>[4x]MGSDKIHHHHHHMIDLRSDTVTKPTEEMRKAMAQAEVGDDVYGEDPTINELERLAAETFGKEAALFVPSGTMGNQVSIMAHTQRGDEVILEADSHIFWYEVGAMAVLSGVMPHPVPGKNGAMDPDDVRKAIRPRNIHFPRTSLIAIENTHNRSGGRVVPLENIKEICTIAKEHGINVHIDGARIFNASIAS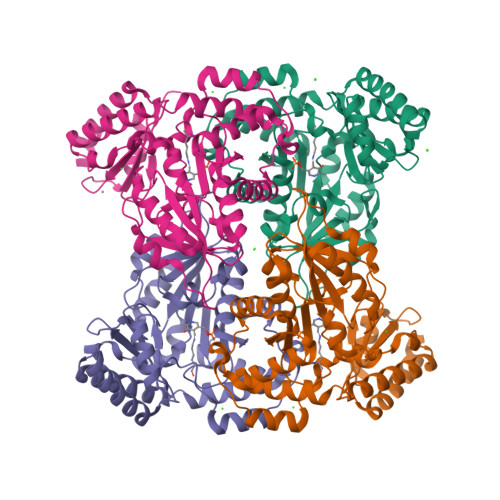GVPVKEYAGYADSVMFCLSKGLCAPVGSVVVGDRDFIERARKARKMLGGGMRQAGVLAAAGIIALTKMVDRLKEDHENARFLALKLKEIGYSVNPEDVKTNMVILRTDNLKVNAHGFIEALRNSGVLANAVSDTEIRLVTHKDVSRNDIEEALNIFEKLFRKFS>MKLIVGMTGATGAPLGVALLQALREMPNVETHLVMSKWAKTTIELETPYSARDVAALADFSHNPADQAATISSGSFRTDGMIVIPCSMKTLAGIRAGYADGLVGRAADVVLKEGRKLVLVPREMPLSTIHLENMLALSRMGVAMVPPMPA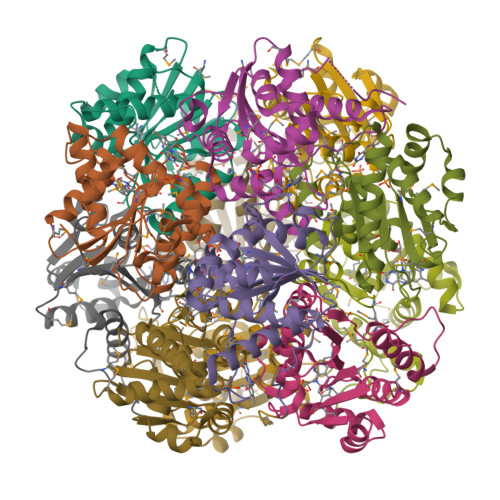FYNHPETVDDIVHHVVARVLDQFGLEHPYARRWQGLPQARNFSQENE[4x]> IESIIKTATDTVKSEINAELGVVPSLNAVETGATSNTEPEEAIQTRTVINQHGVSETLVENFLSRAALVSKRSFEYKDHTSSAAQTDKNFFKWTINTRSFVQLRRKLELFTYLRFDAEITILTTVAVNGSSNNTYVGLPD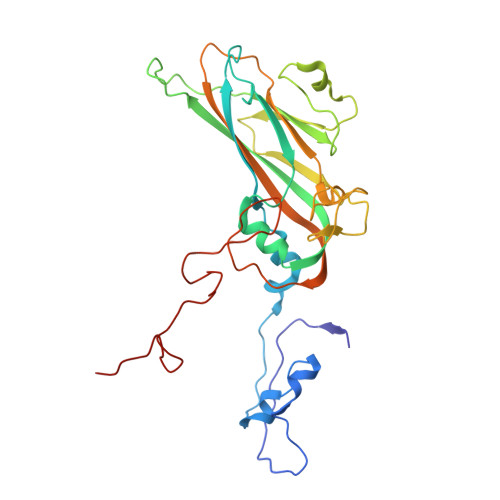LTLQAMFVPTGALTPEKQDSFHWQSGSNASVFFKISDPPARMTIPFMCINSAYSVFYDGFAGFEKSGLYGINPADTIGNLCVRIVNEHQPVGFTVTVRVYMKPKHIKAWAPRPPRTLPYMSIANANYKGKGRAPNALNAIIGNRDSVKTMPHNIVTT>[2x]GSHGMVSVSEIRKAQRAEGPATILAIGTANPANCVEQSTYPDFYFKITNSEHKTELKEKFQR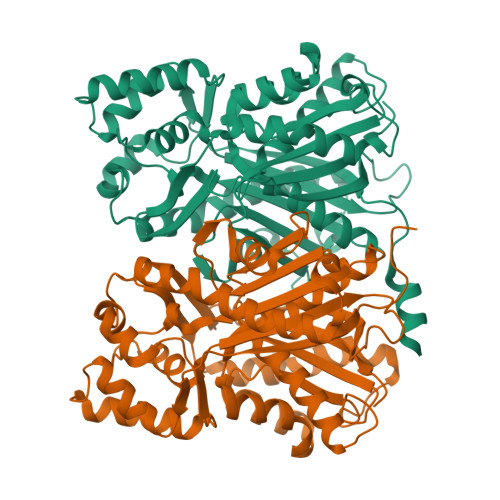MCDKSMIKRRYMYLTEEILKENPNVCEYMAPSLDARQAMLAMEVPRLGKEAAVKAIKEWGQPKSKITHLIVCSTTTPDLPGADYQLTKLLGLRPYVKRVGVFQHGCFAGGTVLRLAKDLAENNKGARVLVVCSEVTAVTFRGPSDTHLDSLVGQALFGDGAAALIVGSDPVPEIEKPIFEMVWTAQTIAPDSEGAIDGHLREAGLTFHLKGAVPDIVSKNITKALVEAFEPLGISDYNSIFWIAHPGGPAILDQVEQKLALKPEKMNATREVLSEYGNMSSACVLFILDEMRKKSTQNGLKTTGEGLEWGVLFGFGPGLTIETVVLRSVAI However, only a dozen of the corresponding gene products were biochemically characterized including the tetrachloroethene RDase (PceA) of the epsilonproteobacterium Sulfurospirillum multivorans. PceA was described to mediate the reductive dehalogenation of chlorinated and brominated ethenes or propenes. The crystal structure of PceA showed the norpseudo-B12 non-covalently bound in its ‘base-off’ conformation deeply inside the protein. The two [4Fe–4S] clusters of PceA connect the surface and cobamide cofactor at distances short enough to allow intramolecular electron transfer to the active site and potentially also from the proximal Fe–S cluster to the substrate.

PceA dehalogenated 4-iodophenol (4-IP) three times faster than 4-BP, while 4-chlorophenol (4-CP) was not converted. Activity measurements using 4-CP, 4-BP and 4-IP showed an enhanced reduction rate with decreasing electronegativity of the halogen substituent from chloride to iodide. The position and orientation of the analogues 4-CP, 4-BP and 4-IP in the active site of substrate–enzyme complexes is thereby identical, independent of the type of halogen. It has to be concluded that exclusively the differences in the energy of the various carbon–halogen bonds determine the displacement or continuance of the substituent.

>[2x]AEKEKNAAEIRQQFAMTAGSPIIVNDKLERYAEVRTAFTHPTSFFKPNYKGEVKPWFLSAYDEKVRQIENGENGPKMKAKNVGEARAGRALEAAGWTLDINYGNIYPNRFFMLWSGETMTNTQLWAPVGLDRRPPDTTDPVELTNYVKFAARMAGADLVGVARLNRNWVYSEAVTIPADVPYEQSLHKEIEKPIVFKDVPLPIETDDELIIPNTCENVIVAGIAMNREMMQTAPNSMACATTAFCYSRMCMFDMWLCQFIRYMGYYAIPSCNGVGQSVAFAVEAGLGQASRMGACITPEFGPNVRLTKVFTNMPLVPDKPIDFGVTEFCETCKKCARECPSKAITEGPRTFEGRSIHNQSGKLQWQNDYNKCLGYWPESGGYCGVCVAVCPFTKGNIWIHDGVEWLIDNTRFLDPLMLGMDDALGYGAKRNITEVWDGKINTYGLDADHFRDTVSFRKDRVKKS> MTKYKYTVEESERFNKHGIDLTVYG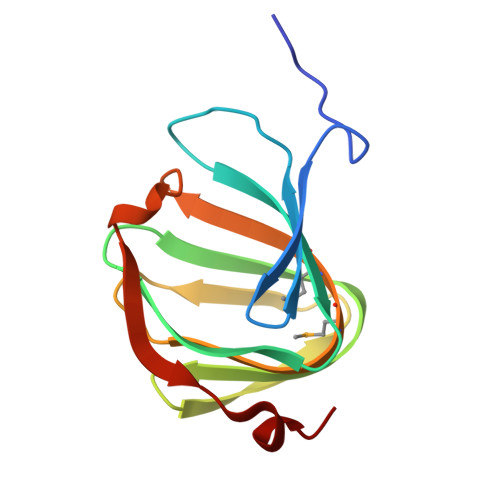QVDPSATVVRVSVERGHFQEFFNVRSSYTYYVVSGQGVFYLNSEAVPAGATDLITVPPNTRIHYFGSMEMVLTVAPAFNEQDERHVRFISESESPY> ANCRILLTPLNERDEQRGYSTQGLKRLSGTAKLNPRLGFTRTQFVQELPRQQKGMSISGYQPKLQLVLDEGEFRVVDHQGNFILKPSPADFPGLAENEHATMTLMSRLGFDVPVHGLLSFAPQSEEELEYAFVIRRYDRDNKGLPVHQEQLDGAMQITDKYGKTGNDNEQYVSYETLARFLVAHVNDNIAFKIDLFRRIVYAWLLGNNDMHLRNFGLVYSDGLTPALAPVYQFVSVAPY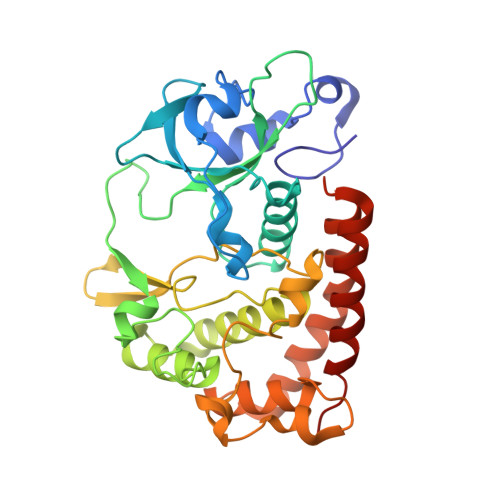PEYFYSNYLALPLLTREEGGRELAPGFHSDYGEYIGQDFLLLGESMGLAPRLLEKLFQDIRKENAIVMETYEQSFMTQDHIQAVLQCYRHRLGLLHHHHHH1-PALMITOYL-2-LINOLEOYL-SN-GLYCERO-3-PHOSPHOCHOLINE | C42 H80 N O8 P | 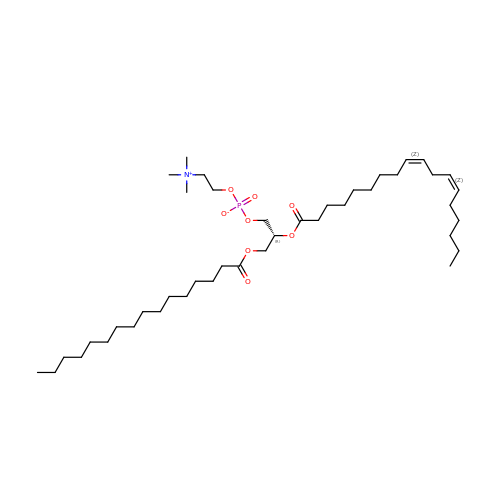JLPULHDHAOZNQI-ZTIMHPMXSA-N1-{4-amino-2-[(ethylamino)methyl]-1H-imidazo[4,5-c]quinolin-1-yl}-2-methylpropan-2-ol 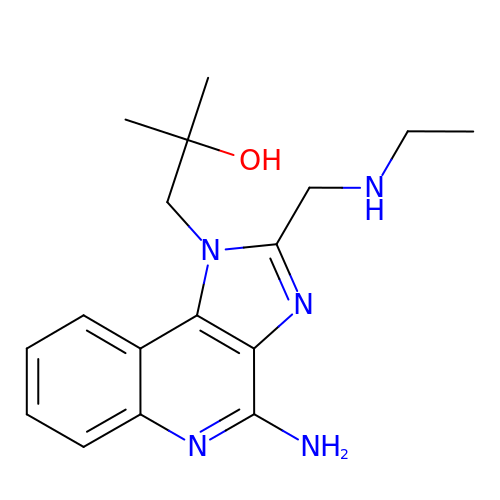| C17 H23 N5 O | FHJATBIERQTCTN-UHFFFAOYSA-N>GPTLVPTKMQVTAPANISASAQTFEVACDYNGAIATLSDDGDMVGTAIVKDGKAIIKLNESIADETNLTLTVVGYNKVTVIKDVKVEGTSIEGRAADKPYTVAVSGKTITVESPAAGLTIFDMNGRRVATAKNRMVFEAQNGVYAVRIATEGKTYTEKVIV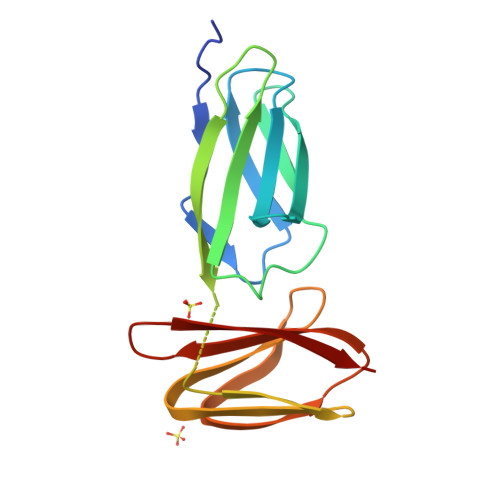K[2x]>[4x]DDDKMNLD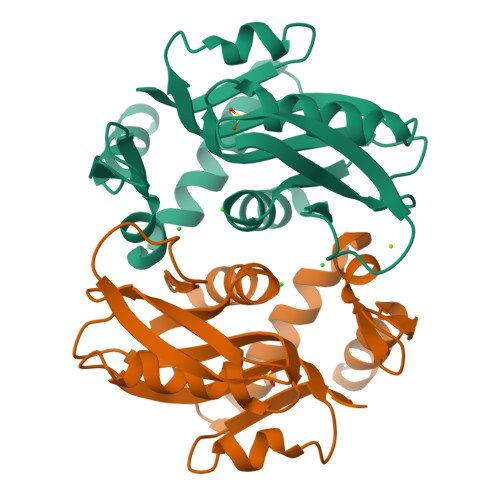FIKSKIAAVPDFPKPGIMFRDITPLLADPQGLRKTAEAMAQELKNKGIQPTIVAGTESRGFIFGVALAEVLGLGFVPVRKPGKLPRATYSVKYDLEYGSDSLEIHQDAFKVTDEVLVVDDLLATGGTAKATVDLIEKTQAKVAGLIFVMELDGLGGREVLAGYNVSALIKF>[3x]MRGSHHHHHHGSPSKVQELS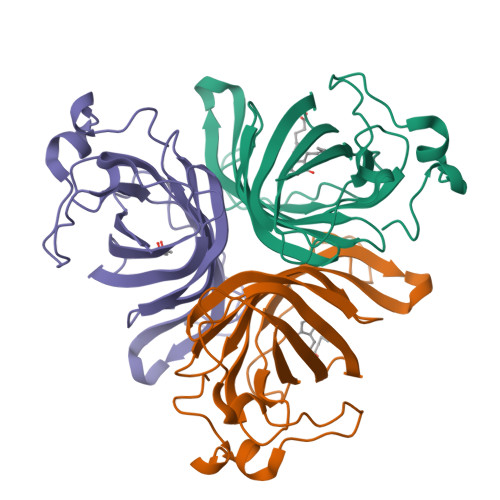VYEINELDRHSPKILKNAFSLMFGLGDLVPFTNKLYTGDLKKRVGITAGLCVVIEHVPEKKGERFEATYSFYFGDYGHLSVQGPYLTYEDSFLAITGGAGIFEGAYGQVKLQQLVYPTKLFYTFYLKGLANDLPLELTGTPVPPSKDIEPAPEAKALEPSGVISNYTN> MKLLRRIAAPAIALGIAMSTIVTPSTAGAAEVTPADVAGDTALSTISDSAPADEASAPRWRAHVNAADERVKEMWAYSPSMDRNVPLVVITADESAGPRPVIYLLNGGDGGEGAANWVMQTDVLDFYLEKNVNVVIPMEGKFSYYTDWVEENASLGGKQMWETFLVKELPGPLEEKLNTDGQRAIAGMSMSATTSLLFPQHFPGFYDAAASFSGCAATSSLLPWEYLKLTLDRGNATPEQMWGPRGGEYNIYNDALINSDKLRGTELYVSNASGLAGEWESVDSPRFEGLNQQVQSIAMAETVVTGGIIEAATNKCTHDLKAKLDSAGIPADWNLRPTGTHSWGWWQDDLRGSWTTFARAFELEA

Protein mycoloylation is a newly characterized post-translational modification (PTM) specifically found in Corynebacteriales, an order of bacteria that includes numerous human pathogens. Recently, some mycomembrane proteins including PorA have been unambiguously shown to be covalently modified with mycolic acids in the model organism Corynebacterium glutamicum by a mechanism that relies on the mycoloyltransferase MytC. The mycolate transfer from TMM to various acceptors are known to be catalyzed by mycoloyltransferases (Myts), a family of enzymes specifically present in all members of Corynebacteriales. Porin mycoloylation is abolished in a mutant strain deleted for the gene encoding MytC, one of the six mycoloyltransferases described in C. glutamicum proving that this protein is either directly or indirectly involved in this modification.

Here, to further explore the mechanism and the specificity of protein mycoloylation, we took profit of our TMM analog library to obtain crystals from MytC trapped in its acyl-enzyme state. We tested both the TMM-C13:0 (analog 2), a water-soluble analog of TMM and TMP (analog 6), the previously characterized inhibitor of the reaction. The protein crystallized in the very rare space group F23 and the asymmetric unit contained one copy of MytC with a solvent content of 49%. The Polder map shows that S189 Oγ atom forms an ester bond with the carbonyl of the analog. This structure will be further referred to as the MytC-acyl enzyme (MytC with catalytic S189 esterified). Electron density in the MytC-acyl enzyme was well defined for residues 30 to 363, except for the segment between 283 to 287. The meromycolic chain of the mycolate C13:0 is directed towards the exit of the active site cave, while the α-chain is more deeply buried and establishes hydrophobic interactions with residues of MytC α11 helix. The β-hydroxyl group, a determinant for PorA modification by MytC, does not establish polar interactions with MytC. The MytC catalytic triad residues S189, H341, and E310 are clearly in an inactive configuration: the H341 Nδ is at a distance of 14.8 Å from the S189 Oγ and 13.5 Å from the E310 Oε1. In the apoform, a small helix (η3) contained between residues 270 to 280, is positioned between S189, H341 and E310, blocking the active site pocket. This helix unfolds in the MytC-acyl enzyme structure to form an irregular loop, becoming part of the active site wall, thereby providing space for the binding of the α-alkyl moiety of the mycolate chain C13:0.>MALGSLLALLALLLLWGAVAEGPAKKVLTLEGDLVLGGLFPVHQKGGPAEDCGPVNEHRGIQRLEAMLFALDRINRDPHLLPGVRLGAHILDSCSKDTHALEQALDFVRASLSRGADGSRHICPDGSYATHGDAPTAITGVIGGSYSDVSIQVANLLRLFQIPQISYASTSAKLSDKSRYDYFARTVPPDFFQAKAMAEILRFFNWTYVSTVASEGDYGETGIEAFELEARARNISVATSEKVGRAMSRAAFEGVVRALLQKPSARVAVLFTRSEDARELLAASQRLNASFTWVASDGWGALEEVVAGSEGAAEGAITIELASYPISDFASYFQSLDPWNNSRNPWFREFWEQRFRCSFRQRDCAAHSLRAVPFEQESKIMFVVNAVYAMAHALHNMHRALCPNTTRLC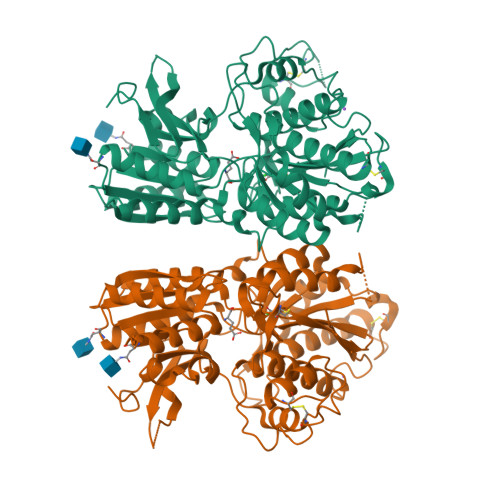DAMRPVNGRRLYKDFVLNVKFDAPFRPADTHNEVRFDRFGDGIGRYNIFTYLRAGSGRYRYQKVGYWAEGLTLDTSLIPWASPSAGEGHHHHHH[2x]> GSGGIEGGSMGTIKSLLPKSEDDLDSEMAVESWSGDKLK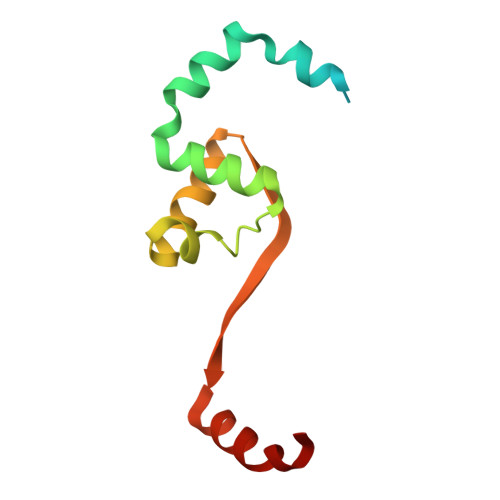NEVEQLAPEEQEILTAIYTGITSLELPGMMGMDIDEVEKVLEKLIDQGFLDLVRIRKETDLTEKGRAVTNFIITNF> GSDDDNPTVDPANIDYTPENASSWHNYMRNVAALLKTDATNLYNAWNSSYKGGESYASLFKAHSGSPYASALSCVEEIVDKCAEIANEVGTAKIGDPYNLYKAGNTEEALYAVESWYSWHSRDDYTNNIYSIRNAYYGSLDGNINANSLSTVIAGANSSLD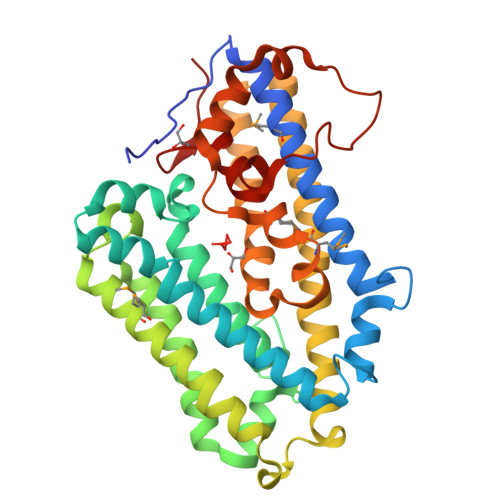TKIKNAIQKAAKAIQDIPQPFRNHIPSNETVAAMDACAELESILKNDLKSYIANNSNNINTDAVLNPVVTQYVDAVVVPTYKSLKEKNDALYNAVIVLADNPSNSAFETACDAWITAREPWEKSEAFLFGPVDEMGLDPNMDSWPLDQNAIVQILNSQSWSDLEWSEGDDEAAVESAQNVRGFHTLEFLLYKNGEPRKVQ>[2x]GENGESVVVLDKYGYPILYAPEEIGEEKEYSKYEDVVIEWNPSVTPVQIEKNYEVKFDVRQVKLRPPKVKNGSGKEGEIIVEAYASLFKSRLSKLKRILRENPEISNVVDIGKLNYVSGDEEVTIIGLVNSKRETNRGLIFEVEDKTGIVKVFLPKDSED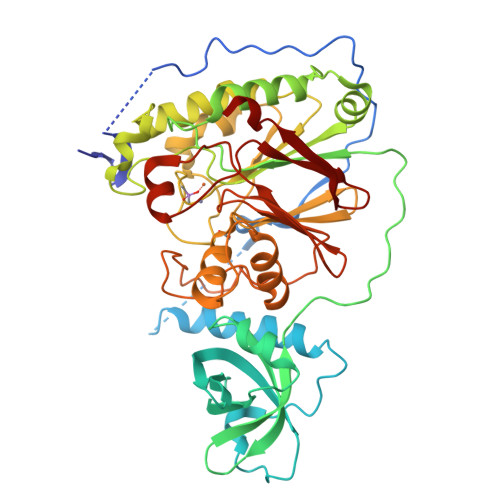YREAFKVLPDAVVAFKGFYSKKGIFFANKFYLPDVPLYRKQKPPLEEKVYAILISDIHVGSREFCEKAFLKFLEWLNGHVESKEEEEIVSRVKYLIIAGDVVDGIGIYPGQYSDLVIPDIFDQYEALANLLANVPEHITMFIGPGNADAARPAIPQPEFYKEYAKPIYKLKNAIIISNPAVIRLHGRDFLIAHGRGIEDVVSFVPGLTHHKPGLPMVELLKMRHLAPTFGGKVPIAPDPEDLLVIEEVPDLVQMGHVHVYDAVVYRGVQLVNSATWQAQTEFQKMVNIVPTPAKVPVVDVESARVVKVLDFSGWC All classes of bacterial IgA1Ps cleave host IgA1 within the heavy-chain (HC) hinge region, the linker connecting the IgA1 constant fragment (Fc) to its antigen binding region (Fab), leaving the light chain (LC) intact while separating the Fc and Fab. The overall structure reveals that S. pneumoniae IgA1P is a multi-domain enzyme, broadly comprised of N-terminal (NTD; residues 665–1070), middle (MD; 1071–1611), and C-terminal domains (CTD; 1612–1963). The active site is formed between the MD and CTD domains that bifurcate the Zn-coordinating residues of the HEMTH motif (residues 1604–1608 in the MD) and a downstream E (E1628 in the CTD). We have determined the structure of a member of the M26 metalloprotease IgA1P subfamily of bacterial IgA1Ps both in isolation as well as in complex with its human IgA1 substrate and solved its structure with a neutralizing mAb that provides insight into blocking S. pneumoniae IgA1P activity.

Thus, we focused our cryo-EM studies on a construct of IgA1P spainning residues 665–1963 that could be excised from its MBP tag and had comparable cleavage to the full-length IgA1P. A defining feature of this S. pneumoniae β-helix is both its relatively small size and the lack of protruding secondary structure elements from within the domain itself. The IgA1P MD and CTD have no structural similarity to any known protein to date, as indicated by the lack of structural similarity using DALI searches. Despite the unique structural folds of the IgA1P MD and CTD, the S. pneumoniae IgA1P active site comprises catalytically important residues within similar positions to that of the prototypical metalloprotease, thermolysin, which supports a conserved catalytic mechanism that is consistent with our previous biochemical studies. Specifically, three side chains from IgA1P H1604, H1608, and the downstream E1628 coordinate the Zn atom and are homologous with thermolysin residues H142, H146, and E166, respectively. The Zn both polarizes the carbonyl group of the scissile peptide bond and activates the nucleophilic water molecule that is deprotonated by a fourth residue, E1605 (E143 in thermolysin). Thus, it is the NTD that repositions from a “closed” state in the absence of substrate to an “open” state allowing for binding of the IgA1 hinge region. The number of interactions between the IgA1P NTD and MD are diminished upon this rearrangement, providing for an energetic rationale for why the enzyme “snaps” back after product release.

> TEPEKKLELRNVSDIELYSQTNGTYRQHVSLDGIPENTDTYFVKVKSSAFKDVYIPVASITEEKRNGQSVYKITAKAEKLQQELENKYVDNFTFYLDKKAKEENTNFTSFSNLVKAINQNPSGTYHLAASLNANEVELGPDERSYIKDTFTGRLIGEKDGKNYAIYNLKKPLFENLSGATVEKLSLKNVAISGKNDIGSLANEATNGTKIKQVHVDGVLAGERGVGGLLAKADQSSIAESSFKGRIVNTYETTDAYNIGGLVGHLTGKNASIAKSKATVTISSNTNRSDQTVGGLAGLVDQDAHIQNSYAEGDINNVKHFGKVAGVAGYLWDRTSGEEKHAGELTNVLSDVNVTNGNAITGYHYTGMKVANTFSSKANRVFNVTLEKDEVVSKESFEERGTMLDASQIVSKKAEINPLTLPTVEPLSTSGKKDSDFSKIAHYQANRALVYKNIEKLLPFYNKSTIVKYGNLVKENSLLYQKELLSAVMMKDDQVITDIVSNKQTANKLLLHYNDHSSEKFDLKYQTDFANLAEYNLGNTGLLYTPNQFLYDRDSIVKEVLPELQKLDYQSDAIRKTLGISPEVKLTELYLEDQFSKTKQNLGDSLKKLLSADAGLAADNSVTRGYLVDKIKNNKEALLLGLTYLERWYNFNYGQVNVKDLVMYHPDFFGKGNTSPLDTLIELGKSGFNNLLAKNNVDTYGISLASQHGATDLFSTLEHYRKVFLPNTSNNDWFKSETKAYIVEEKSTIEEVKTKQGLAGTKYSIGVYDRITSATWKYRNMVLPLLTLPERSVFVISTMSSLGFGAYDRYRSSDHKAGKALNDFVEENARETAKRQRDHYDYWYRILDEQSREKLYRTILLYDAYKFGDDTTSGKATAEAKFDSSNPAMKNFFGPVGNKVVHNQHGAYATGDGVYYMSYRMLDKDGAITYTHEMTHDSDQDIYLGGYGRRNGLGPEFFAKGLLQAPDQPSDATITINSILKHSKSDSTEGSRLQVLDPTERFQNAADLQNYVHNMFDLIYMMEYLEGQSIVNKLSVYQKMAALRKIENKYVKDPADGNEVYATNVVKELTEAEARNLNSFESLIDHNILSAREYQSGDYERNGYYTIKLFAPIYSALSSEKGTPGDLMGRRIAYELLAAKGFKDGMVPYISNQYEEDAKQQGQTINLYGKERGLVTDELVLKKVFDGKYKTWAEFKTAMYQERVDQFGNLKQVTFKDPTKPWPSYGTKTINNVDELQALMDQAVLKDAEGPRWSNYDPEIDSAVHKLKRAIFKAYLDQTNDFRSSI>[3x]PFLELDTNLPANRVPAGLEKRLCAAAASILGKPADRVNVTVRPGLAMALSGST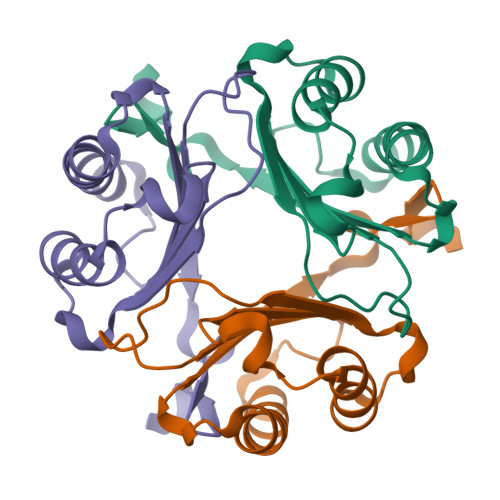EPCAQLSISSIGVVGTAEDNRSHSAHFFEFLTKELALGQDRILIRFFPLESWQIGKIGTVMTFL> MAENTEPRIGVFVCHCGTNIAGSMSIDDVVNYAKTLPYVAVADQYQYMCSTPGQKKIDDAIKEYNLTGVVVAACSPRLHEPTFRTATKEGGLNPFRFEMANIREQNSWVHMHGMWDEATQKAKDQVRMAVAKAAKLEDLVPKSVPVEKTAMVVGGGVAGMQAALDLASAGIKTYLIERTPTIGGRMSQLDKTFPTLDCSQCILTPKMVDVGRHPNIEMMTYTEVEKVEGYIGNFDVTL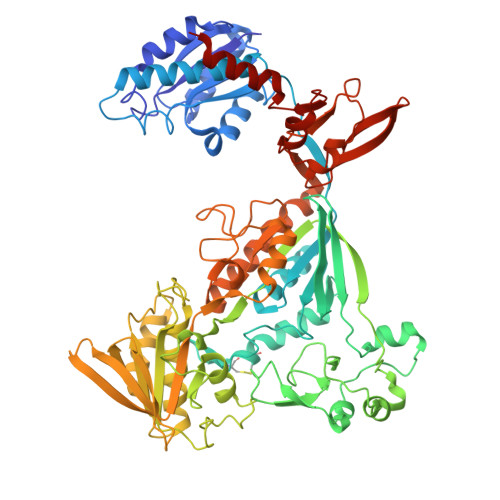RKKARGVLTPTEATAKGIVGGGCNGCGDCSAVCPVIKPNPFEMGMAPRKAIYIYHAQVMPLIYTVDFDSCVKCGLCVEACGDKKAIDLEMQDEFITVKVGTAVLATGYELFPIENKREWGYKQFDNVINALEFERLICASGPTGGHLVRPSDGKTPMKVGFVLCAGSRDNTGIGKPYCSRFCCMYSLKHAHQIMEKIPGAVAYLFYMDIRSFGKMYEEFYYRIQHEGAKFIRGRVANVLEDKETKNLHVFTEDTLLGRPVDVEVDLLVLAAAVQPNEGANELRKKFGVSASQDGWMLEAHPKLNPCGTTTAGVFLAGVCQGPKDIPDTVAQAEGAASAASIPIHMGEVELEPYFAMCIDELCAGCGMCVNLCPYSALSLGEKNGRTVMVVTEAKCKGCGTCGGFCPGGAIKMQHFTTPQIVAQIDAFFAGGEQ>[2x]MFENITAAPADPILGLADLFRADERPGKINLGIGLYYDETGKIPVLTSVKKAEQYLLENETTKLYLGIDGIPEFGRCTQELLFGKGSALINDKRARTAQTPGGSGALRVAADFLAKNTSVKRVWVSNPSWPNHKSVFNSAGLEVREYAYYDAENHTLDFDALINSLNEAQAGDVVLFHGCCHNPTGI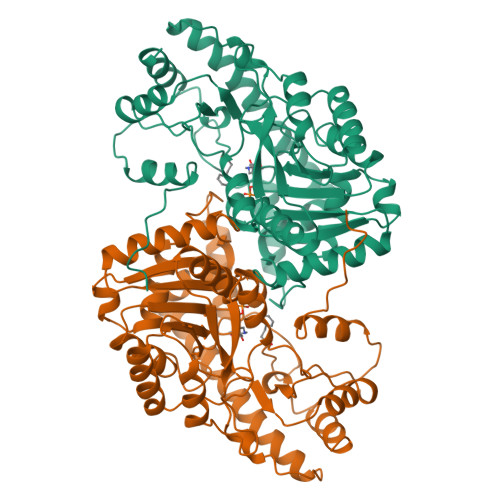DPTLEQWQTLAQLSVEKGWLPLFDFAYQGFARGLEEDAEGLRAFAAMHKELIVASSYSKNFGLYNERVGACTLVAADSETVDRAFSQMKAAIRANYSSPPAHGASVVATILSNDALRAIWEQELTDMRQRIQRMRQLFVNTLQEKGANRDFSFIIKQNGMFSFSGLTKEQVLRLREEFGVYAVASGRVNVAGMTPDNMAPLCEAIVAVL>[2x]GCANNQTNASQPAEKNEKTEMKDDFAKLEEQFDAKLGIFALDTGTNRTVTYRPDERFAFASTIKALTVGVLLQQKSIEDLNQRITYTRDDLVNYNPITEKHVDTGMTLKELADASLRYSDNTAQNLILKQIGGPESLKKELRKIGDEVTNPERFEPELNEVNPGETQDTSTARALATSLQAFALEDKLPSEKRELLIDWMKRN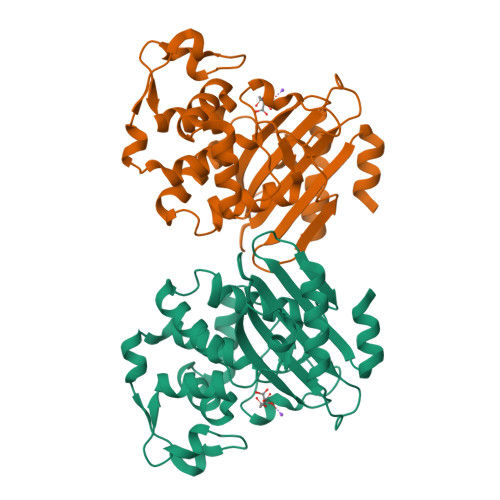TTGDALIRAGVPEGWEVADKTGAGSYGTRNDIAIIWPPKGDPVVLAVLSSRDKKDAKYDDKLIAEATKVVLKALNMNGK>[2x]MAAESVRVAVRCRPFNQREKDLNTTLCVGMTPNVGQVNLNAPDGAAKDFTFDGAYFMDSTGEQIYNDIVFPLVENVIEGYNGTVFAYGQTGSGKTFSMQGIETIPAQRGVIPRAFDHIFTATATTENVKFLVHCSYLEIYNEEVRDLLGADNKQKLEIKEQPDRGVYVAGLSMHVCHDVPACKELMTRGFNNRHVGATLMNKDSSRSHSIFTVYVEGMTETGSIRMGKLNLVDLAGSERQSKTGATGDRLKEATKINLSLSALGNVISALVDGKSKHIPYRDSKLTRLLQDSLGGNTKTIMIACVSPSSDNYDETLSTLRYANRAKNIKNKPTINEDPLEHHHHHH

OSM‐3 belongs to the homodimeric kinesin‐2 subfamily and is the Caenorhabditis elegans homologue of human KIF17. Similar to KIF17, OSM‐3 is involved in intraflagellar transport in the distal part of the cilium, and both proteins are autoinhibited at the resting state. The OSM‐3 motor domain shows the typical kinesin fold, with a central eight‐stranded β‐sheet surrounded by 3 α‐helices on either side. We have determined the structure of the motor domain of OSM‐3 either bound to ADP or to AMPPNP, or devoid of a nucleotide.

We reasoned that, by adding apyrase just before setting up crystallization trials, nucleotide‐free OSM‐3 might be incorporated and stabilized in a crystal before denaturing. Indeed, OSM‐3 crystals diffracting X‐rays up to a resolution of 2.3 Å were obtained in these conditions. The structure was solved by molecular replacement taking that of ADP‐OSM‐3 as a search model and there are two virtually identical kinesin molecules per asymmetric unit (rmsd 0.44 Å; 308 Cα atoms aligned). The electron density maps indicated that the nucleotide‐binding site was indeed devoid of a nucleotide. Instead, an electron density was located close to the missing ADP β phosphate, as observed in other structures of nucleotide‐free kinesins. In the case of OSM‐3, this density is well accounted for by a sulfate ion that likely comes from the crystallization solution. The structure of nucleotide‐free OSM‐3 is however very similar to that of the ADP form, with an rmsd ranging from 0.49 (chain B) to 0.55 Å (chain A; 304 Cαs aligned in both cases). In particular, the L9 and L11 loops, belonging to the Switch 1 and Switch 2 regions, respectively, are disordered and the neck linker is docked onto the motor domain core. Relatedly, the structure of nucleotide‐free OSM‐3 is closer to that of ADP‐kinesin‐1 with a docked neck linker than to tubulin‐bound nucleotide‐free kinesin‐1. Finally, we note that the overall temperature factor of OSM‐3 was unexpectedly high (about 87 Å2) for a 2.3 Å resolution structure, likely reflecting further the instability of this kinesin in the absence of a nucleotide.>VPMGKFAMYPDWQPDADFIRLAALWGVALREPVTTEELASFIAYWQAEGKVFHHVQWQQKLARSLQIGRAS[5x]

The second primosome is the oriC-independent PriA primosome, which requires PriA to recognise the n′-pas (primosome assembly site) and initiate the primosome assembly. In general, the PriA binds to n′-pas while assisted by the auxiliary PriB, PriC, DnaT, to recruit the DnaB, DnaC and DnaG. In summary, the ssDNA binding protein DnaT, the N-terminal end of which is crucial for PriB binding, exists as a trimer in solution. Biochemical and structural information shows that the DnaT can cooperatively bind to ssDNA to form rod-like nucleoprotein filaments, which indicate that the DnaT-ssDNA complex might function as a scaffold during primosome assembly.

Except for the dT10 ssDNA ligand, there are five molecules that display as a C-shaped helical assembly in one asymmetry unit. The protomers are similar to one other, having a root mean square deviation for the Cα atoms of no more than 0.3 Å; each protomer contains a three-helix bundle that has the α3 helix flanked by the α1 and α2 helixes. The five molecules are mediated through dimeric interfaces between each two adjacent subunits. Taking the A and B interface as an example, the interaction interface is mediated mainly through the α2 helix in subunit A and the L1 loop and the α1 and α3 helixes in subunit B using hydrogen bonds and hydrophobic residues. The ssDNA binds in a hydrophobic and positively charged cavity at the junction between different subunits of the DnaT84–153, with each protomer binding to a 2-base unit using the α2 and α3 helixes. The phosphodiester backbone is recognised mainly by Lys133, Lys143, and Arg146 through hydrogen bonds, while the 2-thymine-base unit is stabilised through the hydrophobic centre formed by Phe124, Tyr127, Trp128, Phe135, Arg146, Ile150 and Gly151. The Tyr127 and Ile150 stack against the two bases from each side of the two bases directly. Each base of the 2 bases stacks against the other, and all of the 5 DnaT84–153 subunits bind to the 2 bases in a similar way. The 2.83 Å DnaT84–153–dT10 complex structure showed a unique ssDNA binding mode that is different from any of the known RNA binding motifs.> AMGSQSLYREIHQLISFKDVLPDKNLLPDWSSNKNPCTFDGVTCRDDKVTSIDLSSKPLNVGFSAVSSSLLSLTGLESLFLSNSHINGSVSGFKCSASLTSLDLSRNSLSGPVTTLTSLGSCSGLKFLNVSSNTLDFPGKVSGGLKLNSLEVLDLSANSISGANVVGWVLSDGCGELKHLAISGNKISGDVDVSRCVNLEFLDVSSNNFSTGIPFLGDCSALQHLDISGNKLSGDFSRAISTCTELKLLNISSNQFVGPIPPLPLKSLQYLSLAENKFTGEIPDFLSGACDTLTGLDLSGNHFYGAVPPFFGSCSLLESLALSSNNFSGELPMDTLLKMRGLKVLDLSFNEFSGELPESLTNLSASLLTLDLSSNNFSGPILPNLCQNPKNTLQELYLQNNGFTGKIPPTLSNCSELVSLHLSFNYLSGTIPSSLGSLSKLRDLKLWLNMLEGEIPQELMYVKTLETLILDFNDLTGEIPSGLSNCTNLNWISLSNNRLTGEIPKWIGRLENLAILKLSNNSFSGNIPAELGDCRSLIWLDLNTNLFNGTIPAAMFKQSGKIAANFIAGKRYVYIKNDGMKKECHGAGNLLEFQGIRSEQLNRLSTRNPCNITSRVYGGHTSPTFDNNGSMMFLDMSYNMLSGYIPKEIGSMPYLFILNLGHNDISGSIPDEVGDLRGLNILDL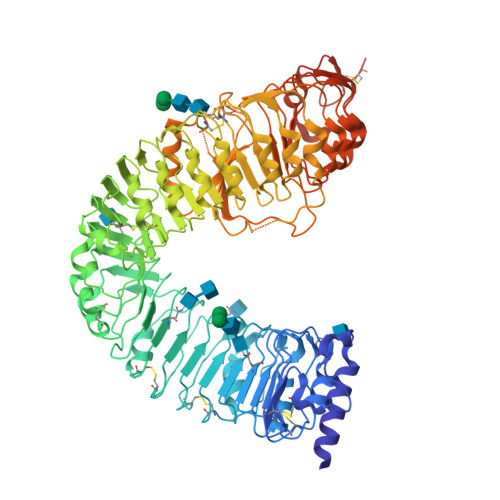SSNKLDGRIPQAMSALTMLTEIDLSNNNLSGPIPEMGQFETFPPAKFLNNPGLCGYPLPRCDPSNADGYAHHQRSHGRRLENLYFQGA>MPFSDFVLALKDNPYFGAGFGLVGVGTALAMARKGAQLGLVAFRRHYMITLEVPARDRSYAWLLSWLTRHSTRTQHLSVETSYLQHESGRISTKFEFIPSPGNHFIWYQGKWIRVERNRDMQMVDLQTGTPWESVTFTALGTDRKVFFNILEEARALALQQEEGKTVMYTAVGSEWRTFGYPRRRRPLDSVVLQQGLADRIVKDIREFIDNPKWYIDRGIPYRRGYLLYGPPGCGKSSFITALAGELEHSICLLSLTDSSLSDDRLNHLLSVAPQQSLVLLEDVDAAFLSRDLAVENPIKYQGLGRLTFSGLLNALDGVASTEARIVFMTTNYIDRLDPALIRPGRVDLKEYVGYCSHWQLTQMFQRFYPGQAPSLAENFAEHVLKATSEISPAQVQGYFMLYKNDPMGAVHNIESLRPRDHHHHHH[7x]

The human AAA-ATPase Bcs1L translocates the fully assembled Rieske iron-sulfur protein (ISP) precursor across the mitochondrial inner membrane, enabling respiratory Complex III assembly. Bcs1L is a membrane-bound oligomer, with each subunit consisting of an N-terminal TM segment, a middle Bcs1-specific domain, and a C-terminal AAA domain that is highly distinct, forming a clade of its own in the broad AAA protein family. Here, we captured Bcs1L conformations by cryo-EM during active ATP hydrolysis in the presence or absence of ISP substrate. In contrast to the threading mechanism widely employed by AAA proteins in substrate translocation, subunits of Bcs1L alternate uniformly between ATP and ADP conformations without detectable intermediates that have different, co-existing nucleotide states, indicating that the subunits act in concert.

Two independent ATP states were identified in this work: ATP state-1 and ATP state-2. Another smaller EM dataset was collected with similar conditions but using a different grid type, leading to a uniform ATP-bound reconstruction at 3.46 Å (C1) and 3.02 Å (C7) resolution, respectively. Surprisingly, this map has the membrane cavity better ordered with the TM helices resolved (ATP state-2). To obtain the best resolution for the TM region of mBcs1L structures, we performed 3D reconstructions in C7 symmetry for the two ATP-bound maps (ATP state-1 and ATP state-2) and the ADP-bound map. For example, in our ADP and ATP state-2 maps, we could trace the density all the way to the N-terminus of mBcs1L, depicting the structures of the entire N-termini exposed to the IMS to form the IMS seal, the complete TM helices, and additionally the apparent ordered densities that could be modeled as lipid molecules circling the base of the membrane basket. By contrast, the ATP state-2 reveals a near-complete structure of the TM region, showing a similar membrane-embedded basket encircled by TM helices as in the ADP state (right). For the ATP state-2, the TM helices pass through the MIM at an apparent tilting angle ϕ of 60°, leaning down more towards the membrane plane compared to the ADP state that has a tilting angle of 70°. This difference in ϕ results in a shallower TM basket and a slightly more opened IMS-seal with a diameter of ~13 Å, which is consistent with a previous observation by AFM showing the IMS seal undergoing an up-and-down movement during turnover. The EM density for TM region of mBcs1L structure in the ATP state-2 is the least well-defined with reduced local resolution, indicating elevated mobility in this region. In the ATP state-2, the β-sheet I tilts away from the MIM, unpacking the seal loops and opening the Matrix-seal.> GQVIARHKVREFNINPVNTPTKSKLHPSVFYDVFPGDKEPAVLS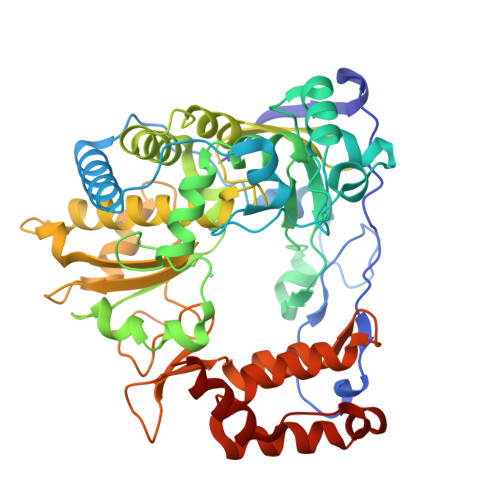DNDPRLEVKLTESLFSKYKGNVNTEPTENMLVAVDHYAGQLLSLDIPTSELTLKEALYGVDGLEPIDITTSAGFPYVSLGIKKRDILNKETQDTEKMKFYLDKYGIDLPLVTYIKDELRSVDKVRLGKSRLIEASSLNDSVNMRMKLGNLYKAFHQNPGVLTGSAVGCDPDVFWSVIPCLMDGHLMAFDYSNFDASLSPVWFVCLEKVLTKLGFAGSSLIQSICNTHHIFRDEIYVVEGGMPSGCSGTSIFNSMINNIIIRTLILDAYKGIDLDKLKILAYGDDLIVSYPYELDPQVLATLGKNYGLTITPPDKSETFTKMTWENLTFLKRYFKPDQQFPFLVHPVMPMKDIHESIRWTKDPKNTQDHVRSLCMLAWHSGEKEYNEFIQKIRTTDIGKCLILPEYSVLRRRWLDLFHHHHHH>SPFHLNDAVAIVTGAAAGIGRAIAGTFAKAGASVVVTDLKSEGAEAVAAAIRQAGGKAIGLECNVTDEQHREAVIKAALDQFGKITVLVNNAGGGGPKPFDMPMSDFEWAFKLNLFSLFRLSQLAAPHMQKAGGGAILNISSMAGENTNVRMASYGSSKAAVNHLTRNIAFDVGP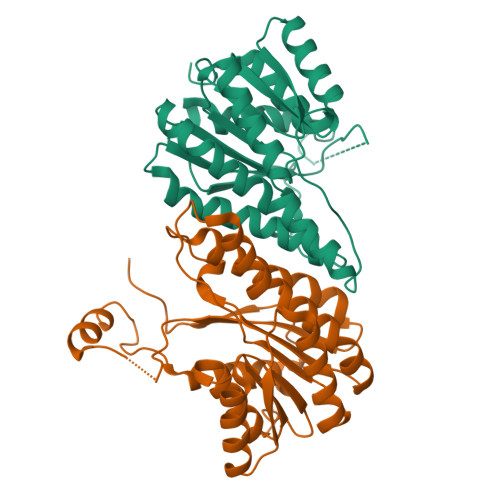MGIRVNAIAPGAIKTDALATVLTPEIERAILKHKPLGRLGEAQDIANAALFLCSPAAAWISGQVLTVSGGGVQE[12x]>[2x]QAISEKDRGNGFFKEGKYERAIECYTRGIAADGANALLPANRAMAYLKIQKYEEAEKDCTQAILLDGSYSKAFARRGTARTFLGKLNEAKQDFETVLLLEPGNKQAVTELSKIKKELIEKGHWDDVFLDSTQRQNVVKPIDNPPHPGSTKPL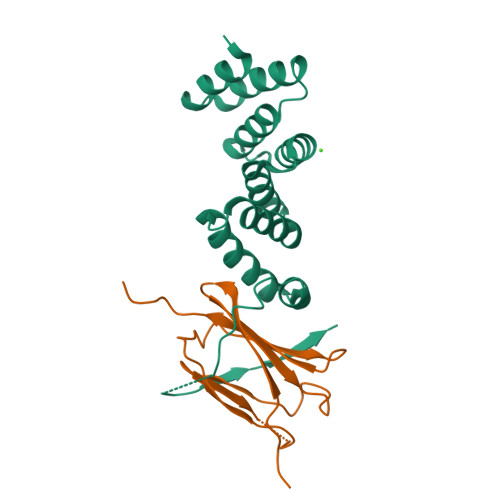KKVIIEETGNLIQ;>GPHMGRAESGPEKPHLNLWLEAPDLLLAEVDLPKLDGALGLSLEIGENRLVMGGPQQLYHLDAYIPLQINSHESKAAFHRKRKQLMVAMPLLPVPS[2x]>[2x]MTIEELKTRL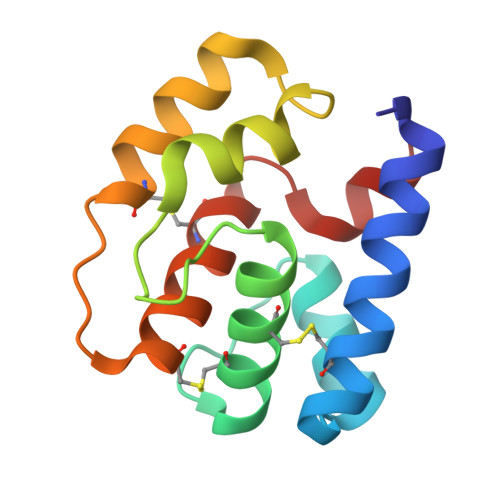HTEQSVCKTETGIDQQKANDVIEGNIDVEDKKVCLYCECILKNFNILDKNNVFKPQGIKAVMELLIDENSVKQLVSDCSTISEENPCLKASKLVQCVSKYKTMKSVDFL>VTAYEEIVCQVFAAVLDRSDVTADADFFALGGHSLLSLRVVARLRALLGVDVGVRDLFEAPTPAALAARLTTQTGRRPAVTRRGPDAPPVLSHFQRRLWLIEQVYQTRGAYNVPLAVHVSDRLDLDVLRAAVRDLVARHEVLRTLVRSSDDGPDPVLLAPEDAAVDVAEVQAAGPVADLLAELTAQPFDLATQIPLRVRMITGEQVDGCVLLLVCHHIAADEWSFAPLLRDLDTAYRARAAGRAPDWEPLPAQYSDYAATLHDWLGEATDPASPLRRQLDYWQHALQDLPDELDLPTDRPRPATASHRGGLARAELPPELVEAVRRLAAQHGVTVFMVVQAAVAVLLHRLGAGDDIPLGSPVADRADEAVHDTVGFFLNTLVLRVNLSGNPTFADLLDRVRAVDLEAFARADAPFDAVVDTVKPPRAVSRHPLFQTMVSYQRRPSDVDRLFGAATRLVEVPLDTAKFDLEFAFIEDGHGGAHIALNYA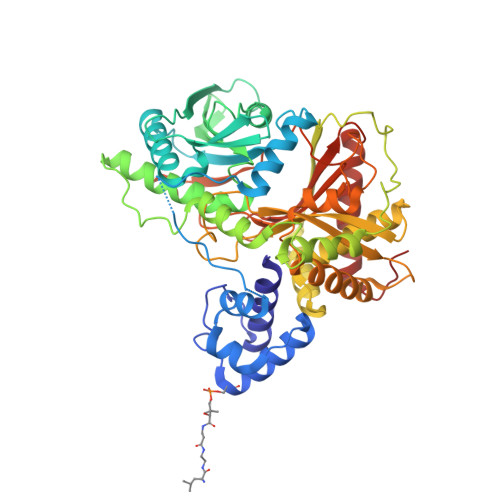ADLFDHDSAEQLVARLRTVLEHACADPCRPVA[2x]>[3x]MLPRETDEEPEEPGRRGSFVEMVDNLRGKSGQGYYVEMTVGSPPQTLNILVDTGSSNFAVGAAPHPFLHRYYQRQLSSTYRDLRKGVYVPYCQGKWEGELGTDLVSIPHGPNVTVRANIAAITESDKFFINGSNWEGILGLAYAEIARPDDSLEPFFDSLVKQTHVPNLFSLQLCGAGFPLNQSEVLASVGGSMIIGGIDHSLYTGSLWYTPIRREWYYEVIIVRV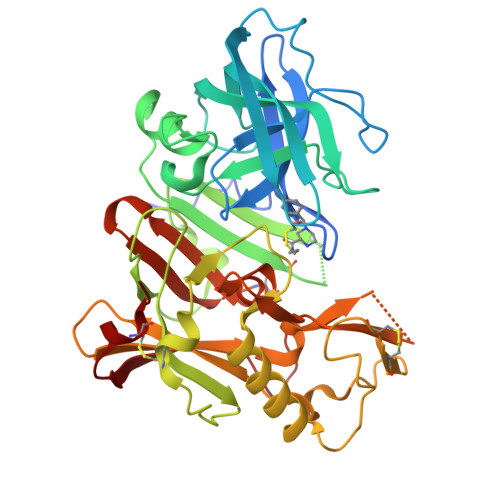EINGQDLKMDCKEYNYDKSIVDSGTTNLRLPKKVFEAAVKSIKAASSTEKFPDGFWLGEQLVCWQAGTTPWNIFPVISLYLMGEVTNQSFRITILPQQYLRPVEDVATSQDDCYKFAISQSSTGTVMGAVIMEGFYVVFDRARKRIGFAVSACHVHDEFRTAAVEGPFVTLDMEDCGYN> MQQFPQFHVKSGLQIKKNAIIDDYKVTSQVLGLGINGKVLQIFNKRTQEKFALKMLQDCPKARREVELHWRASQCPHIVRIVDVYENLYAGRKCLLIVMECLDGGELFSRIQDRGDQAFTEREASEIMKSIGEAIQYLHSINIAHRDVKPENLLYTSKRPNAILKLTDFGFAKETTSHNSLTTPCYTPYYVAPEVLGPEKYDKSCDMWSLGVIMYILLCGYPPFYSNHGLAISPGMKTRIRMGQYEFPNPEWSEVSEEVKMLIRNLLKTE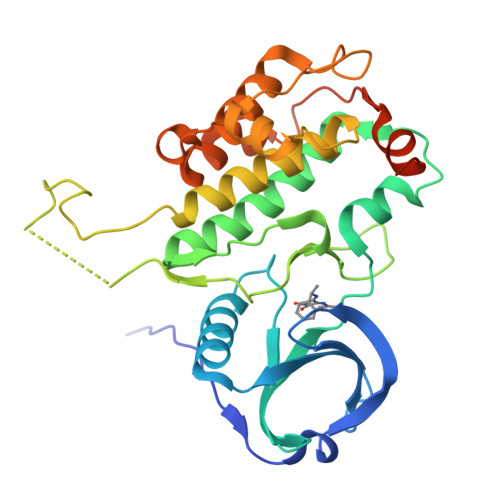PTQRMTITEFMNHPWIMQSTKVPQTPLHTSRVLKEDKERWEDVKEEMTSALATMR> MKFALQINEGPYQHQASDSAYQFAKAALEKGHEIFRVFFYHDGVNNSTRLTTPPQDDRHIVNRWAELAEQYELDMVVCVAAAQRRGIVDEGEASRNGKDATNIHPKFRISGLGQLVEAAIQAD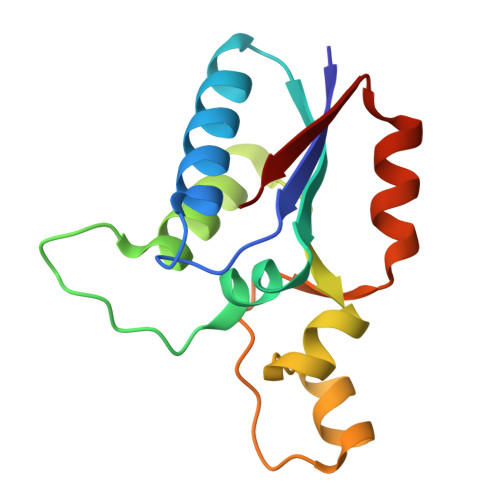RLVVFGD>[4x]ASDHQTQAGK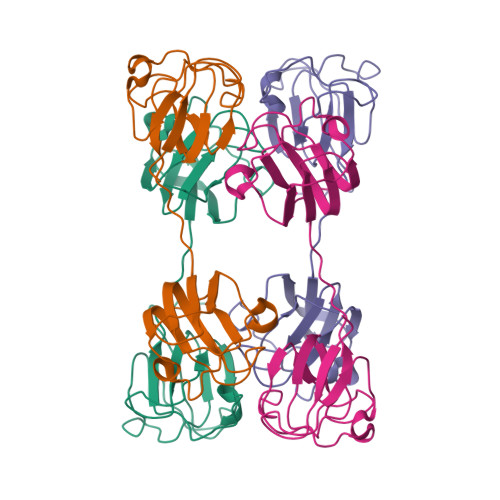PQPLNPKIIIFEQENFQGHSHELNGPCPNLKETGVEKAGSVLVQAGPWVGYEQANCKGEQFVFEKGEYPRWDSWTSSRRTDSLSSLRPIKVDSQEHKITLYENPNFTGKKMEVIDDDVPSFHAHGYQEKVSSVRVQSGTWVGYQYPGYRGLQYLLEKGDYKDSGDFGAPQPQVQSVRRIRDMQWHQRGAFHPSS> MLRGTRGFLAVSPGVGIAPETTPVKYTPMMLNIQNMMWWNGKRNLYRATYREKTWYEISRTGAFTKGRRPVMRQKYSREALQAALAMVPPGFEVADVPRPPQRILAQSEGIVGRWYSNYWTLHSMRYQCLLAGVEWPLGERQRPRTNYDEPFFFADFEESKAIRDYRSRWINVNRSLVGMTKRMKEAEEEARYMQFRKLQ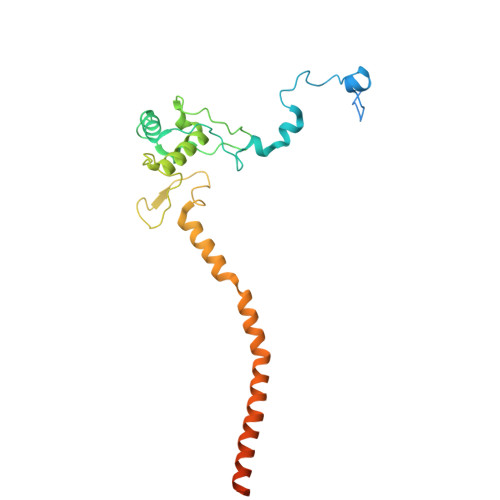DTFWSNRKVLVNRVKSMYNQGARTSAKDMPIKTINIKAFLSE6-cyano-17-(3-pyridyl)-androst-5,16-dien-3-ol | C25 H30 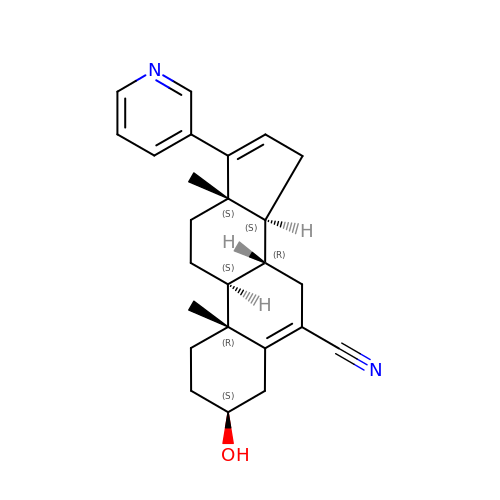N2 O | XMYHDPOWFDNIDA-SQRYLOHGSA-N>[4x]FYHLVDDYGRGNGFFDKFNFFTGDDPT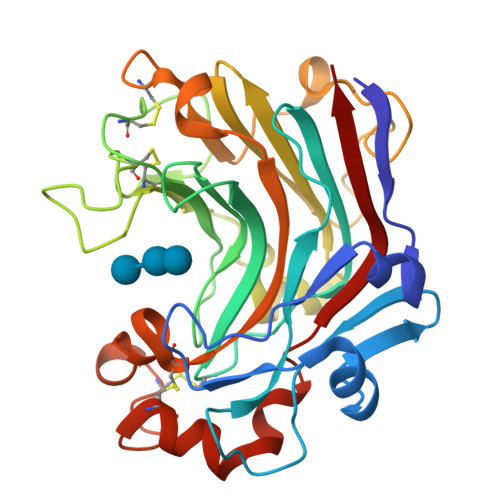HGYVDYVSRDVAAGAGLIGERDGRTYMGVDFTNPASGRGRRSVRLESKNTYEHGLIVIDLAHMPGSVCGTWPAFWTLGTGDWPYGGEIDIIEGVNDNTFNHMVLHTSDGCTIDNDGFTGNLKTSNCYVYAPGQDANAGCGIEATDPNSYGKGFNSIGGGIYATEITPNGISIWFFPRGSEPGDVLGDNPNPANWDTPAAKFAGGGCDWEGKFNAQRLIFDVTFCGDWAGNVWGIGGCASRAANCVDFVRDNPSAFAESYWLVNSLRVYAP>[3x]MDSKDFLARLSLPARLASEQSGVPHHLILAQAALESGWGQRQILRENGEPSYNVFGVKATASWKGPVTEITTTEYENGEAKKVKAKFRVYSSYLEALSDYVALLTRNPRYAAVTTAATAEQGAVALQNAGYATDPNYARKLTSMIQQLKAMSGSHHHHHH

Members of GH family 73 (GH73) are β-N-acetylglucosaminidases that cleave the β-1,4 glycosidic linkage between the N-acetylglucosamine (GlcNAc) and N-acetylmuramic acid (MurNAc) residues of bacterial cell wall peptidoglycan (PG). In some instances, GH73 enzymes are associated with bacterial pathogenicity, for example, LytB being critical for pneumococcal nasal colonization and cell division, Auto for pathogenic listeriosis caused by Listeria monocytogenes, and FlgJ for biogenesis and function of the flagellum, which is a major virulence factor of motile pathogenic bacteria. The domain was found to adopt a lysozyme-like fold common to other GH73 enzymes, which consists of an α-helical subdomain packed against a β-lobe that forms an extended β-hairpin motif. The α-helical domain and β-hairpin of StFlgJGH(151–316) together form a groove-shaped active site, with the α-helical subdomain containing an α-central helix that houses a conserved glutamate general acid/base (E184), and the β-hairpin, in turn, containing a second glutamate residue (E223) previously determined to be required for GH activity.

Next, we determined the crystal structure of the truncated GH domain (StFlgJGH(151–301)) to 2.2 Å resolution to study the active site of StFlgJ in the absence of the C-terminal α-helix. The asymmetric unit contained three copies of the truncated domain. Though the C-terminal α-helix no longer occupied the active site, the catalytic β-hairpin of each domain was found to partly occlude the active site of neighbouring domains in the crystal structure. While this crystal packing did not provide an unobstructed active site, it did impart significant structural order to the β-hairpin. The β-hairpin was found to be located further from the helical domain of the enzyme than any previously reported structure of a GH73 enzyme, including Auto and SpFlgJ. A superposition of StFlgJ with the structures of other GH73 enzymes reveals substantial differences in the position of the β-hairpin harboring the putative catalytic E223 residue. Removing the C-terminal α-helix, however, allowed us to determine a 2.1 Å crystal structure of the domain in which the extended β-hairpin, known to accommodate a second putative catalytic carboxyl group, was well ordered and revealed that the active site of StFlgJ seems capable of opening widely, possibly aiding in substrate capture and turnover. Contrary to our hypothesis, the assays revealed that the StFlgJ GH domain is fully active both with and without the C-terminal α-helix, indicating that the helix does not auto-inhibit StFlgJ GH activity and is likely not functionally equivalent to the N-terminal auto-inhibitory helix of Auto.>[3x]IEVCNKAQQQGPYTLVDYQEKPLNISRIQIKVVKTSVATKGLNFHIGYRAVWRGYCYNGGSLDKNTGCYNDLIPKSPTESELRTWSKSQKCCTGPDAVDAWGSDARICWAEWKMELCHTAKELKKYSNNNHFAYHTCNLSWRCGLKSTHIEVRLQASGGLVSMVAVMP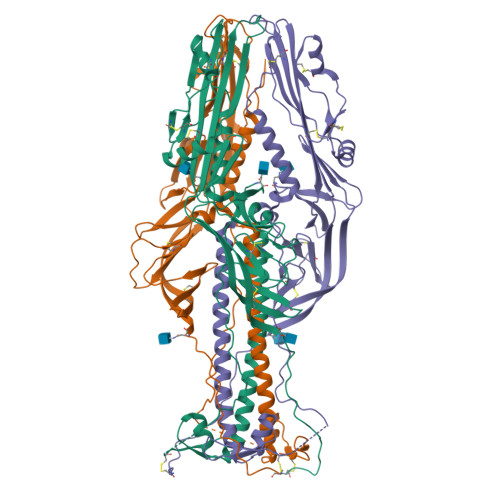NGTLIPIEGTRPTYWTEDSFAYLYDPAGTEKKTESTFLWCFKEHIRPTTELSGAVYDTHYLGGTYDKNPQFNYYCRDNGYYFELPANRLVCLPTSCYKREGAIVNTMHPNTWKVSEKLHSASQFDVNNVVHSLVYETEGLRLALSQLDHRFATLSRLFNRLTQSLAKIDDRLLGTLLGQDVSSKFISPTKFMLSPCLSTPEGDSNCHNHSIYRDGRWVHNSDPTQCFSLSKSQPVDLYSFKELWLPQLLDVNVKGVVADEEGWSFVAQSKQALIDTMTYTKNGGKGTSLEDVLGYPSGWINGKLQG>GCGTATA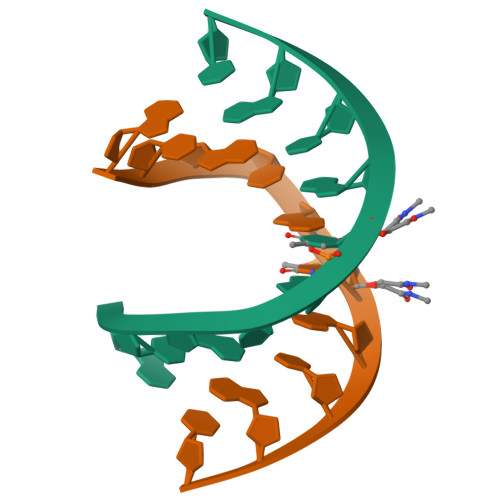CGC[4x]> SNGPQGYASMNGGTTGGAGGRVEYASTGAQIQQLIDNRSRSNNPDEPLTIYVNGTITQGNSPQSLIDVKNHRGKAHEIKNISIIGVGTNGEFDGIGIRLSNAHNIIIQNVSIHHVREGEGTAIEVTDDSKNVWIDHNEFYSEFPGNGDSDYYDGLVDMKRNAEYITVS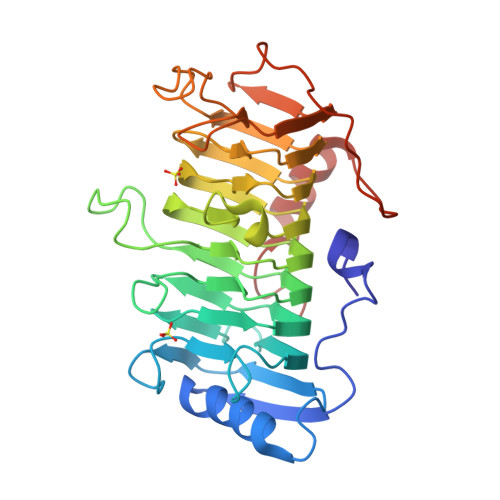WNKFENHWKTMLVGHTDNASLAPDKITYHHNYFNNLNSRVPLIRYADVHMFNNYFKDINDTAINSRVGARVFVENNYFDNVGSGQADPTTGFIKGPVGWFYGSPSTGYWNLRGNVFVNTPNSHLNSTTNFTPPYSYQVQSATQAKSSVEQHSGVGVIN> MADSDINIKTGTTDIGSNTTVKTGDLVTYDKENGMHKKVFYSFIDDKNHNKKLLVIRTKGTIAGQYRVYSEEGAN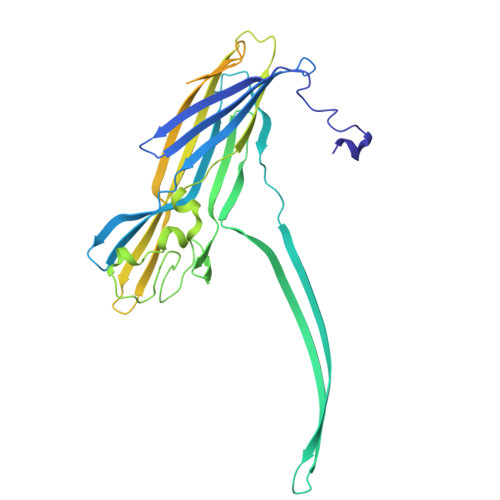KSGLAWPSAFKVQLQLPDNEVAQISDYYPRNSIDTKEYMSTLTYGFNSNVTGDDTGKIGGLIGANVSIGHTLRYVQPDFKTILESPTDKKVGWKVIFNNMVNQNWGPYDRDSWNPVYGNQLFMKTRNGSMKAADNFLDPNKASSLLSSGFSPDFATVITMDRCASKQQTNIDVIYERVRDDYQLHWTSTNWKGTNTKDKWTDRSSERYKIDWEKEEMTNGSSGSVTTLSGLSGEQGPSGDMTTEEDSATHIKFSKRDEDGRELAGATMELRDSSGKTISTWISDGHVKDFYLYPGKYTFVETAAPDGYEVATPIEFTVNEDGQVTVDGEATEGDAHTGGSHHHHHH>[4x]SYYSTLQCRNNHGHCRRLC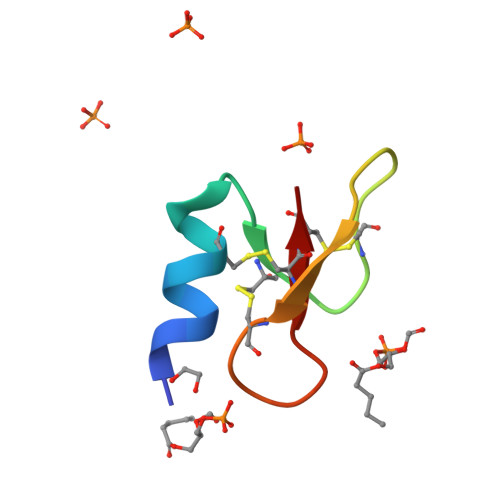FHGEQWIGNCNGRHQHCCK> GHMSETYDFLFKFLVIGNAGTGKSCLLHQFIEKKFKDDSNHTIGVEFGSKIINVGGKYVKLQIWDTAGQERFRSVTRSYYRGAAGALLVYDITSRETYNALTNWLTDARMLASQNIVIILCGNKKD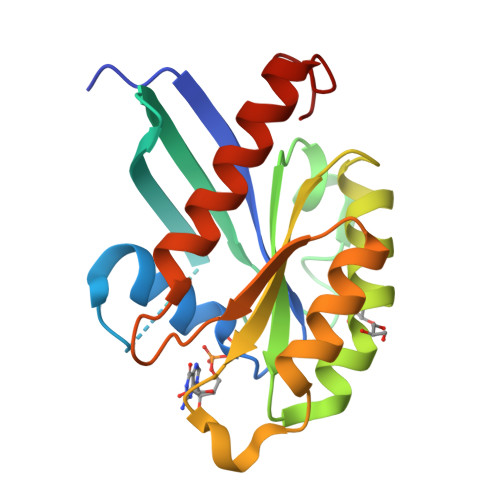LDADREVTFLEASRFAQENELMFLETSALTGENVEEAFVQCARKILNKIESGELDPERMG In the case of σs, a specialized adaptor protein RssB, also referred to as SprE, is not only required for direct recognition of the substrate but also required for its preparation and delivery to the AAA+ protease, ClpXP. RssB is a response regulator (RR), and as such is composed of an N-terminal receiver (REC) domain and a C-terminal output domain (also known as an effector domain). In contrast to most RRs (which contain a DNA binding domain) RssB is linked to a protein binding domain, and as such represents one of the small groups of RRs (~1% of all RRs). Nevertheless, like most RRs, RssB is phosphorylated on a conserved Asp residue (Asp58) within the N-terminal REC domain.

The structure of the RssBC was solved at 2.1 Å by multiple isomorphous replacement. The RssBC domain structure is a mixed α/β-fold with five α-helices and 11 β-strands and can be further divided into a mediator/connector domain (residues 131–163) connecting RssBN with RssBC and the actual C-terminal protein phosphatase (PP2C) domain (residues 164–337). The N-terminal part or connector domain of RssBC comprises three small α-helices (α6–α8) which are arranged with approximate angles of 90 degrees to each other. These helices are connected to the core domain by salt bridges, hydrogen bonds and hydrophobic interactions, but the conformation of the very first α6-helix is likely misaligned due to the absence of the structuring RssBN domain. The α8-helix connects the mediating α-helical elements with the C-proximal and structurally conserved phosphatase domain, which consists of 11 β-strands and two α-helices. The core structure of this domain is formed by a β–sandwich comprising two closely interacting β-sheets. The two β-sheets are stabilized through a hydrophobic core structure formed by conserved aromatic and aliphatic residues. Indeed, the effector domain of RssB exhibits a PPM/PP2C phosphatase fold, however it lacks the active site residues. The conserved residues (between EcRssB and PaRssB) are mostly located in the hydrophobic interface but also include two positively charged surface exposed patches, one of which is centered around the putative phosphatase site that corresponds to the peptides 90 and 91 from the peptide library and hence may play a role in docking to the ZBD of ClpX. Based on our peptide library analysis we propose that the ZBD of ClpX interacts with the α10 helix of RssB.

> MTQPLVGKQILIVEDEQVFRSLLDSWFSSLGATTVLAADGVDALELLGGFTPDLMICDIAMPRMNGLKLLEHIRNRGDQTPVLVISATENMADIAKALRLGVEDVLLKPVKDLNRLREMVFACLYPSMFNSRVEEEERLFRDWDAMVDNPAAAAKLLQELQPPVQQVISHCRVNYRQLVAADKPGLVLDIAALSENDLAFYCLDVTRAGHNGVLAALLLRALFNGLLQEQLAHQNQRLPELGALLKQVNHLLRQANLPGQFPLLVGYYHRELKNLILVSAGLNATLNTGEHQVQISNGVPLGTLGNAYLNQLSQRCDAWQCQIWGTGGRLRLMLSAE> LPGEGTQVHP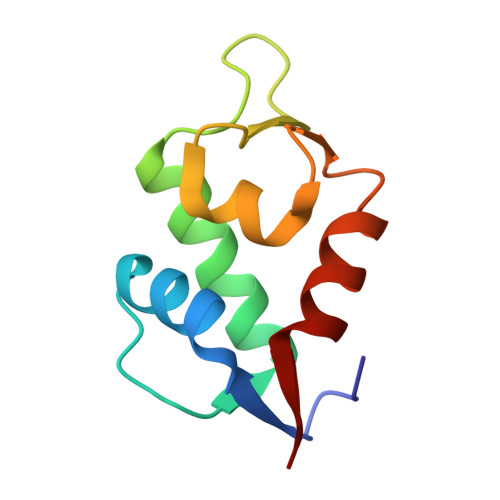RAPLLQILKVAGAQEEVFTVKEVMHYLGQYIMMKQLYDKQRQHIVHCHDDPLGELLEVGSFSVKNPSPLYEMLKRNLVIL;> XLTFXEYWAQLLAAAAAA> HQLQPRRVSFRGEASETLQSPGYDPSRPESFFQQSFQRLSRLGHGSYGEVFKVRSKEDGRLYAVKRSMSPFRGPKDRARKLAEVGSHEKVGQHPCCVRLEQAWEEGGILYLQTELCGPSLQQHCEAWGASLPEAQVWGYLRDTLLALAHLHSQGLVHLDVKPANIFLGPRGRCKLGDFGLLVELGTAGAGEVQEGDPRYMAPELLQGSYGTAADVFSLGLTILEVACNMELPHGGEGWQQLRQGYLPPEFTAGLSSELRSVLVMMLEPDPKLRATAEALLALPVL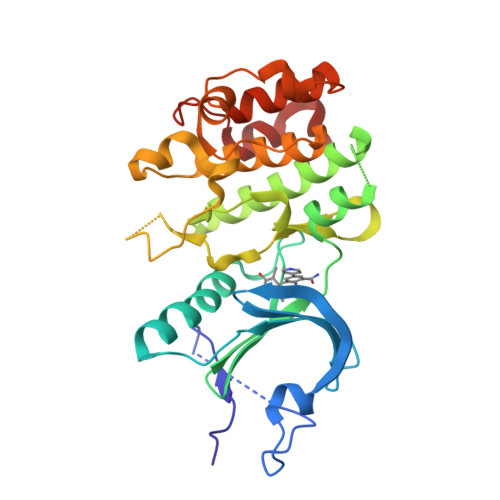RQP>GPMGKMAAAVASLATLAAEPREDAFRKLFRFYRQSRPGTADLGAVIDFSEAHLARSPKPGVPQVVRFPLNVSSVTERDAERVGLEPVSKWRAYGLEGYPGFIFIPNPFLPGCQRHWVKQCLKLYSQKPNVCNLDKHMTKEETQGLWEQSKEVLRSKEVTKRRPRSLLERLRWVTLGYHYNWDSKKYSADHYTPFPSDLAFLSEQVATACGFQGFQAEAGILNYYRLDSTLGIHVDRSELDHSKPLLSFSFGQSAIFLLGGLKRDEAPTAMFMHSGDIMVMSGFSRLLNHAVPRVLPHPDGECLPHCLETPLPAVLPSNSLVEPCSVEDWQVCATYLRTARVNMTVRQVLATGQDFPLEPVE[4x]

AlkB family of 2-oxoglutarate (2OG or α-KG)-dependent oxygenases are evolutionarily conserved and implicated in nucleotide demethylation. Mouse ALKBH1 protein has 389 residues and consists of an N-terminal extension (NTE), a nucleotide-recognition lid (NRL), and a C-terminal double-stranded β helix (DSBH) domain. By establishing a reliable in vitro enzymatic assay, we demonstrated that ALKBH1 prefers bubbled and bulged DNAs, instead of ssDNA or dsDNA substrates. Structural studies of ALKBH1 in substrate-free and a 21-mer bulge DNA-bound state revealed the molecular determinants underlying the observed substrate preference, including unique features of a stretch-out Flip1 motif and a functionally indispensable N-terminal “α1” helix.

Residues 20–358 were modeled based on the electron densities. The DSBH catalytic core of ALKBH1 adopts a typical eight-stranded (I–VIII) jelly-roll fold that contains a major sheet (βI, βVIII, βIII, βVI) and a minor sheet (βVII, βIV, βV and βII) to sandwich Mn(II) and NOG at the active center. The central jelly-roll fold is notably wrapped around and stabilized by additional elements from NTE, NRL and DSBH. In particular, an N-terminal α1 helix of NTE buttresses the minor sheet from the bottom; an extended “coil-sheet” structure of NTE extends the β(V-VI) edge from the back; α3 of NTE and α7 of DSBH organize a helical cluster involving elements α2 and α8, and stack against the major sheet from the top. Moreover, the NRL subdomain composed of elements Flip1 and Flip2 attaches to the β(I) edge of the major sheet, and functionally constitutes the substrate recognition surface along with α1 helix. In contrast, three notably unique structural features to ALKBH1 arise outside the core structure: a far N-terminal α1 helix packed aside the catalytic center, the stretch-out of an extended Flip1, and a long insertion between β(VII) and β(VIII) (INS) that stabilizes Flip1 through helical cluster formation. In contrast, Flip1 of ALKBH1 assumes a fully extended conformation, which is stabilized by extensive hydrophobic and hydrogen-bonding interactions through helical cluster formation among α3 and an “INS” motif, a non-conserved long insertion between β(VII) and β (VIII) unique to ALKBH1. Conceivably, the stretch-out of Flip1 likely leads to the lack of autonomous base-flipping activity of ALKBH1, thus accounting for the observed incompetence of dsDNA demethylation by ALKBH1. The dimension of the substrate channel is ~66 Å in length and ~30 Å in diameter (left and middle), which is well-positioned for duplex substrate recognition of ~20 bp in length (contour length = 68 Å for B-form DNA).> MGSDKIHHHHHHMKISIIGAGSVRFALQLVGDIAQTEELSREDTHIYMMDVHERRLNASYILARKYVEELNSPVKIVKTSSLDEAIDGADFIINTAYPYDPRYHDSGSQRWDEVTKVGEKHGYYRGIDSQELNMVSTYTYVLSSYPDMKLALEIAEKMKKMAPKAYLMQTANPVFEITQAVRRWTGANIVGFCHGVAGVYEVFEKLDLDPEEVDWQVAGVNHGIWLNRFRYRGEDAYPLLDEWIEKKLPEWEPKNPWDTQMSPAAMDMYKFYGMLPIGDTVRNGSWKYHYNLETKKKWFGKFGGIDNEVERPKFHEQLRRARERLIKLAEEVQQNPGMKLTEEHPEIFPKGKLSGEQHIPFINAIANNKRVRLFLNVENQGTLKDFPDDVVMELPVWVDCCGI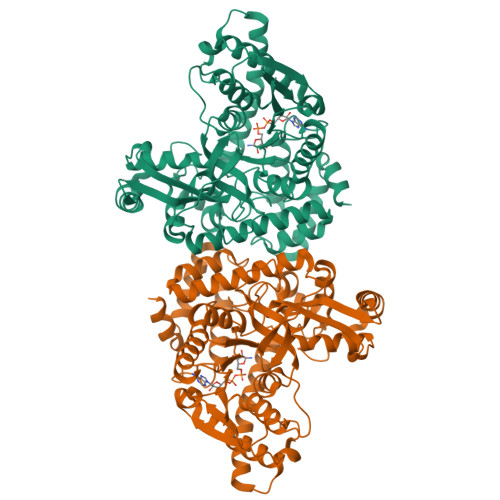HREKVEPDLTHRIKIYLWPRILRMEWNLEAYISRDRKVLEEILIRDPRTKSYEQIVQVLDEIFNLPFNEELRRYYKEKL>MEKNMKFPVVDLSKLNGEERDQTMALINEACENWGFFEIVNHGLPHDLMDKIEKMTKDHYKTCQEQKFNDMLKSKGLDNLETEVEDVDWESTFYVRHLPQSNLNDISDVSDEYRTAMKDFGKRLENLAEDLLDLLCENLGLEK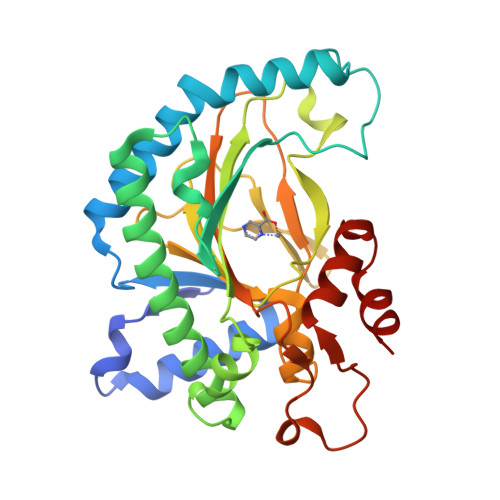GYLKKVFHGTKGPTFGTKVSNYPPCPKPEMIKGLRAHTDAGGIILLFQDDKVSGLQLLKDGDWIDVPPLNHSIVINLGDQLEVITNGKYKSVLHRVVTQQEGNRMSVASFYNPGSDAEISPATSLVEKDSEYPSFVFDDYMKLYAGVKFQPKEPRFAAMK[2x]>MKIKGVNLGNWLVLEKWMSSAIWEGTDAEDEYYLPRGLDSKVYEARIKMHRAEYISERDFARIKAMGFNSVRIPIPYFIYGDRAPFIGCIDELDRAFSWAEKYDLKILIDLHTVPMSQNGFDNGGLSGVCKWAQIPEEVDFVLNLLEKLAKRYGKRKGLLGIEPINQPVSEEMWNDMGVQKRYPPLDKEMAEGSAPISFEWLKGFYDKAADRILPNIDDDKYIVFHDGFRLHAWEEYLTQDRYKGRVILDTHQYLMIAEMLGCEQT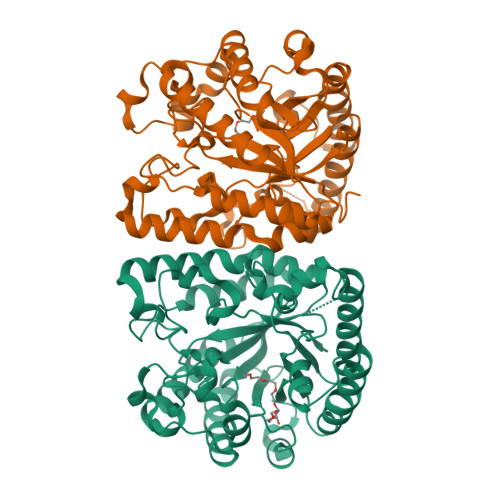LEAYKTFIKEKFEDEITKVEKYVPVVVGQWCIFNSYCVGMDTKGGQSVLNGVDSSDAKGVSDEEKRKVYMELSKAQLKAWDSLSGYFYWTYKMLLDPTNQATWRGWDCWDLAKCVDEGWFPGRVA[2x]> MLKHVAAALLLATAMPVVAQSPAPAAAPAPAARSIAATPPKLIVAISVDQFSADLFSEYRQYYTGGLKRLTSEGAVFPRGYQSHAATETCPGHSTILTGSRPSRTGIIANN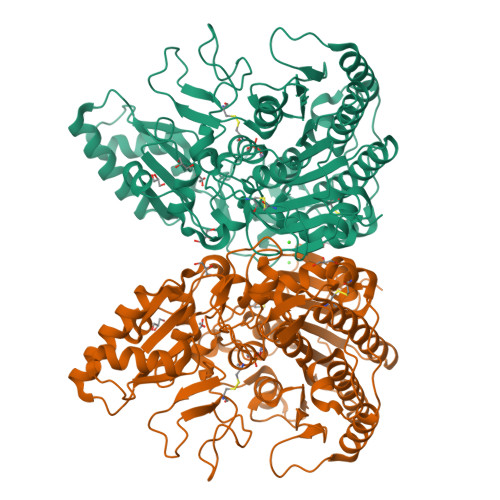WFDLDAKREDKNLYCAEDESQPGSSSDKYEASPLHLKVPTLGGRMKAANPATRVVSVAGKDRAAIMMGGATADQVWWLGGPQGYVSYKGVAPTPLVTQVNQAFAQRLAQPNPGFELPAQCVSKDFPVQAGNRTVGTGRFARDAGDYKGFRISPEQDAMTLAFAAAAIENMQLGKQAQTDIISIGLSATDYVGHTFGTEGTESCIQVDRLDTELGAFFDKLDKDGIDYVVVLTADHGGHDLPERHRMNAMPMEQRVDMALTPKALNATIAEKAGLPGKKVIWSDGPSGDIYYDKGLTAAQRARVETEALKYLRAHPQVQTVFTKAEIAATPSPSGPPESWSLIQEARASFYPSRSGDLLLLLKPRVMSIPEQAVMGSVATHGSPWDTDRRVPILFWRKGMQHFEQPLGVETVDILPSLAALIKLPVPKDQIDGRCLDLVAGKDDSCAGQHHHHHH>[2x]MGTFTSDSASTRFSQAFGIQTGDAVASTITVFQALSIDDQLAVLWYAYTEMGRSITPAATGAARLQ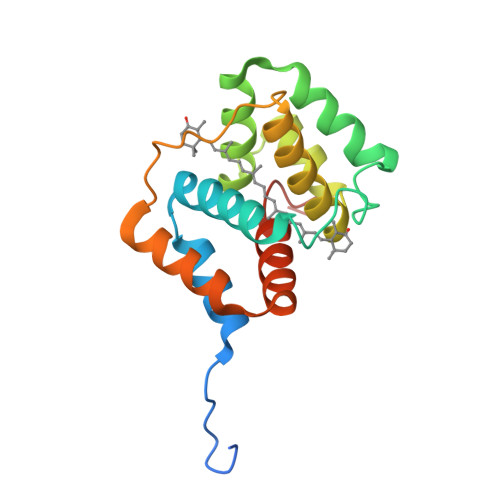LAEGLLNQIKQMSHAEQLQVMRDLAAKNNTQVSRSYGILSNNTKLAFWYELSELMVKGFVVPVPTDYKISRDGSQVLEALKGLDFGQQITVLRKVVADMGVDPLAHHHHHH> AIGEFMVSLPRMVYPQPKVLTPCR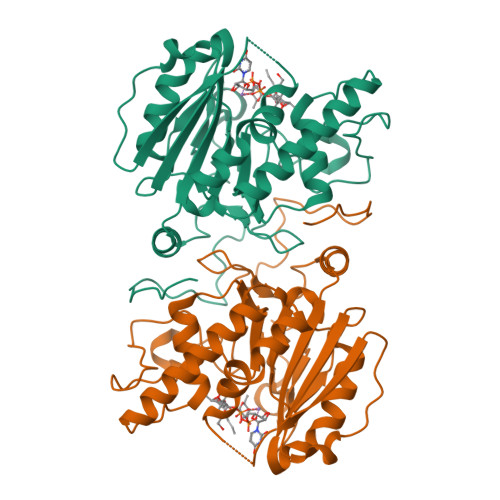KDVLVVTPWLAPIVWEGTFNIDILNEQFRLQNTTIGLTVFAIKKYVAFLKLFLETAEKHFMVGHRVHYYVFTDQPAAVPRVTLGTGRQLSVLEVGAYKRWQDVSMRRMEMISDFCERRFLSEVDYLVCVDVDMEFRDHVGVEILTPLFGTLHPSFYGSSREAFTYERRPQSQAYIPKDEGDFYYMGAFFGGSVQEVQRLTRACHQAMMVDQANGIEAVWHDESHLNKYLLRHKPTKVLSPEYLWDQQLLGWPAVLRKLRFTAVPKNHQAVRNPE> VYELQVQKSVTVQEGLCVLVPCSFSYPWRSWYSSPPLYVYWFRDGEIPYYAEVVATNNPDRRVKPETQGRFRLLGDVQKKNCSLSIGDARMEDTGSYFFRVERGR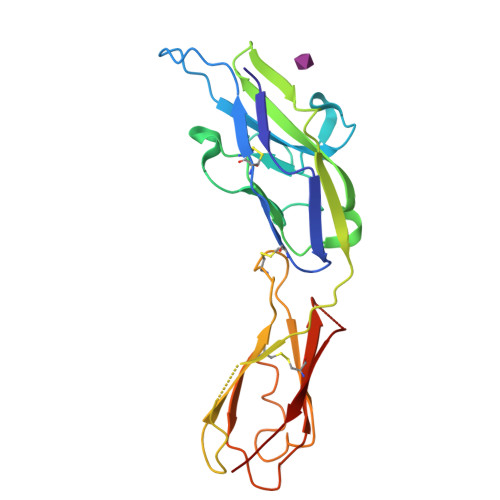DVKYSYQQNKLNLEVTALIEKPDIHFLEPLESGRPTRLSCSLPGSCEAGPPLTFSWTGNALSPLDPETTRSSELTLTPRPEDHGTNLTCQMKRQGAQVTTERTVQLNVS>[4x]LGRHFYVTGPVVRGAGRGGKELGFPTANQYFHDTVALPADGVYAGWLT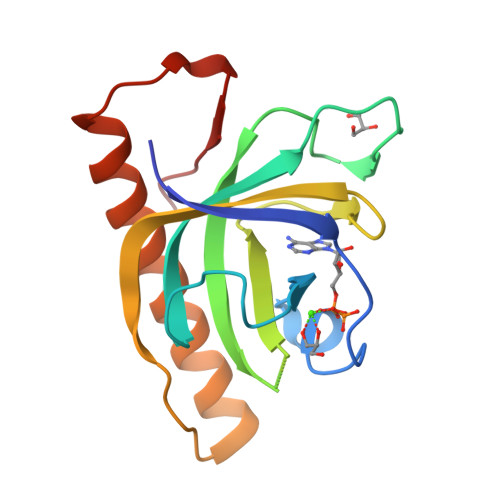ILPTEAPVSGNMEPEVAYAAAISVGTNPTFGDEQRSVESFVLDRDADLYGHDVKVEFVDHVRAMEKFDSVEQLLEVMAKDVQKTRTLLAQDVQAHKMAPETYFLQAES>MGSHHHHHHDITSLYKKAGSAAAVLEENLYFGGSFTMANVNKTPGKTRRAEVAGGGFAGLTAAIALKQNGWDVRLHEKSSELRAFGAGIYLWHNGLRVLEGLGALDDVLQGSHTPPTYETWMHNKSVSKETFNGLPWRIMTRSHLHDALVNRARALGVDISVNSEAVAADPVGRLTLQTGEVLEADLIVGADGVGSKVRDSIGFKQDRWVSKDGLIRLIVPRMKKELGHGEWDNTIDMWNFWPRVQRILYSPCNENELYLGLMAPAADPRGSSVPIDLEVWVEMFPFLEPCLIEAAKLKTARYDKYETTKLDSWTRGKVALVGDAAHAMCPALAQGAGCAMVNAFSLSQDLEEGSSVEDALVAWETRIRPITDRCQALSGDYAANRSLSKGNMFTPAAL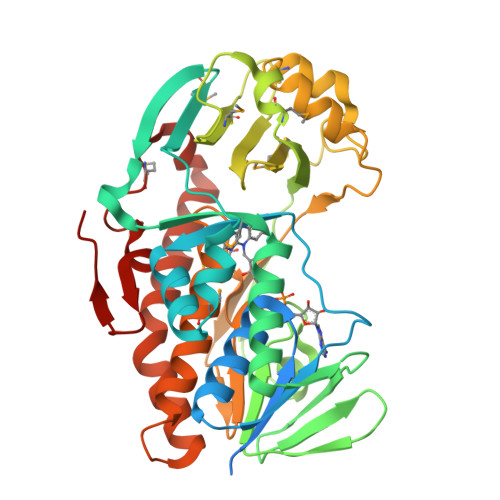EAARYDPLRRVYSWPQ[2x]>PSLSKEAALVHEALVARGLETPLRPPVHEMDNETRKSLIAGHMTEIMQLLNLDLADDSLMETPHRIAKMYVDEIFSGLDYANFPKITLIENKMKVDEMVTVRDITLTSTCESHFVTIDGKATVAYIPKDSVIGLSKINRIVQFFAQRP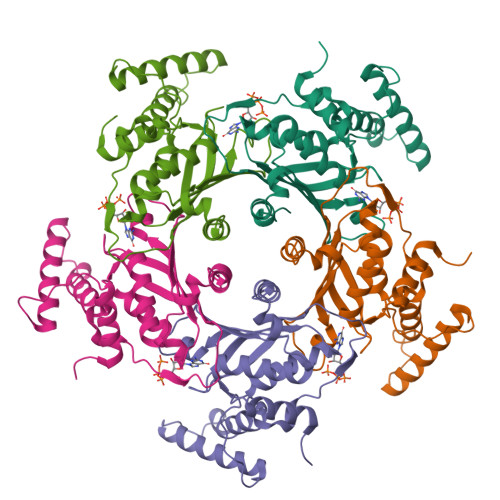QVQERLTQQILIALQTLLGTNNVAVSIDAVHYCVKARGIRDATSATTTTSLGGLFKSSQNTRHEFLRAVRHHN[15x]>[2x]GSHMTVHFIGAGPGAADLITIRGRDLIASCPVCLYAGSLVPEALLAHCPPGAKIVNTAPMSLDAIIDTIAEAHAAGQDVARLHSGDLSIWSAMGEQ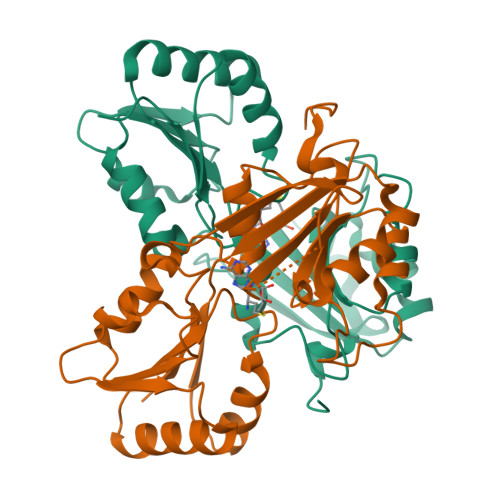LRRLRALNIPYDVTPGVPSFAAAAATLGAELTLPGVAQSVILTRTSGRASAMPAGETLENFARTGAVLAIHLSVHVLDEVVQKLVPHYGEDCPVAIVWRASWPDQRVVRATLATLQTSLGAELERTALILVGRSLATEDFDESRLYAGDYDRRYRPLGTHPRFPEGSE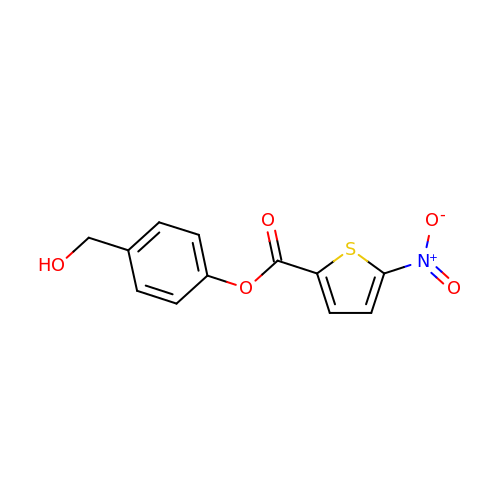[4-(hydroxymethyl)phenyl] 5-nitrothiophene-2-carboxylate | C12 H9 N O5 S | OFKWTDNFZOSQNL-UHFFFAOYSA-N>MLKHIPKNISPDLLKTLMEMGHGDEIVLADANYPSASCANKLIRCDGVNIPELLDSILYLMPLDSYVDSSIQFMNVVSGDDIPKIWGTYRQMIEGHGTDLKTITYLRREDFYERSKKAYAIVATGETS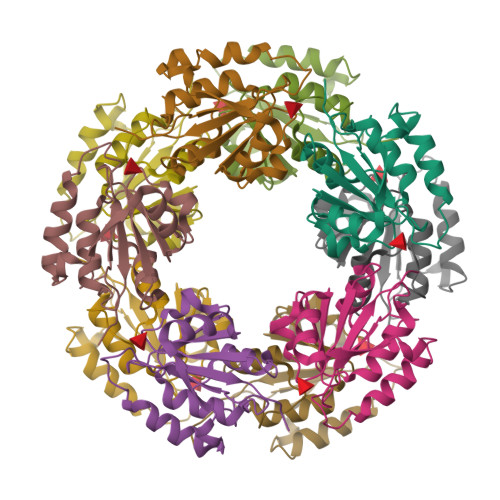LYANIILKKGVVVERENVQ[20x]> GSSSHSMR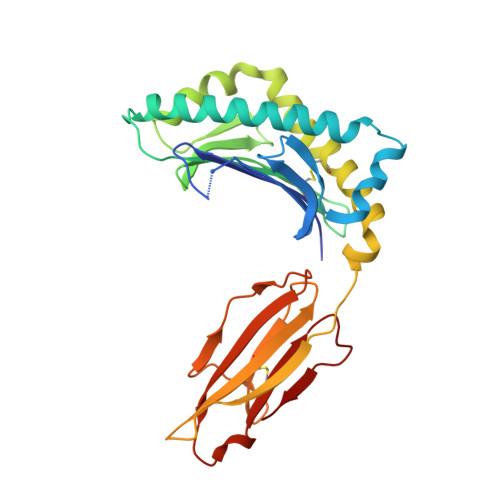YFVTSVSEPGQQVPQFSYVGYVDDQEFVSYNASTRRYLPKVPWISKVEKNDPDYWERNTLYAQGHERSFRDHLATLAEYYNQSGGLHTFQWMYGCELRNDWSKGGYYQYAYDGRDYISLDKDTLTWMAADVPAQNTKRKWDADFRDNEYKKTYLEETCIEWLQRYLNYGKETLLRTEVPEVKVTRKEDYDGMETLICRVGGFYPKDIDIDWTRDGEVWLQDVFHGLVSPNSDGTYYTWRSVKVDPKERERYKCHVEHDGLPNPVDVAW>[2x]APDTSVSNKQNFSTDVIYQIFTDRFSDGNPANNPTGAAFDGSCTNLRLYCGGDWQGIINKINDGYLTGMGITAIWISQPVENIYSVINYSGVNNTAYHGYWARDFKKTNPAYGTMQDFKNLIDTAHAHNIKVIIDFAPNHTSPASSDDPSFAENGRLYDNGNLLGGYTNDTQNLFHHYGGTDFSTIENGIYKNLYDLADLNHNNSSVDVYLKDAIKMWLDLGVDGIRVDAVKHMPFGWQKSFMATINNYKPVFTFGEWFLGVNEISPEYHQFANESGMSLLDYRFAQKARQVFRDNTDNMYGLKAMLEGSEVDYAQVNDQVTFIDNHDMERFHTSNGDRRKLEQALAFTLTSRGVPAIYYGSEQYMSGGNDPDNRARLPSFSTTTTAYQVIQKLAPLRKSNPAIAYGSTHERWINNDVIIYERKFGNNVAVVAINRN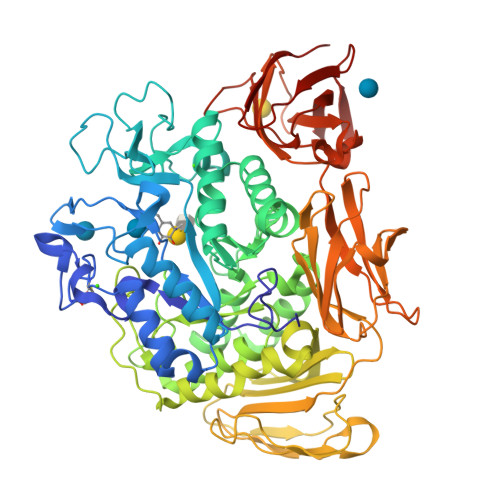MNTPASITGLVTSLPRGSYNDVLGGILNGNTLTVGAGGAASNFTLAPGGTAVWQYTTDATTPIIGNVGPMMAKPGVTITIDGRGFGSGKGTVYFGTTAVTGADIVAWEDTQIQVKIPAVPGGIYDIRVANAAGAASNIYDNFEVLTGDQVTVRFVINNATTALGQNVFLTGNVSELGNWDPNNAIGPMYNQVVYQYPTWYYDVSVPAGQTIEFKFLKKQGSTVTWEGGANRTFTTPTSGTATVNVNWQP> SEFENPLKRLLVPGEEWEFEVTAFYRGRQVFQQTISCPEGLRLVGSEVGDRTLPGWPV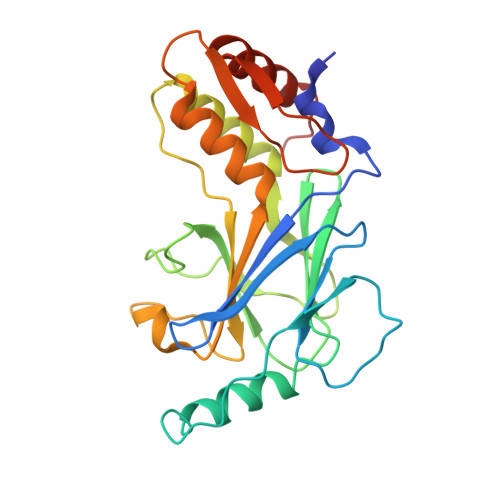TLPDPGMSLTDRGVMSYVRHVLSCLGGGLALWRAGQWLWAQRLGHCHTYWAVSEELLPNSGHGPDGEVPKDKEGGVFDLGPFIVDLITFTEGSGRSPRYALWFCVGESWPQDQPWTKRLVMVKVVPTCLRALVEMARVGGASSLENTVDLHISNSHPLSLTSDQYKAYLQDLVEGMDFQGPGES> EPDIRPCGRSLVIISTLDGRIAALDPENHGKKQWDLDVGSGSLVSSSLSKPEVFGNKMIIPSLDGDLFQWDRDRESMETVPFTVESLLESSYKFGDDVVLVGGKSLTTYGLSAYSGKVRYICSALGCRQWDNDEMEQEEDILLLQRTQKTVRAVGPRSGNEKWNFSVGHFELRYIPDMETRAGFIE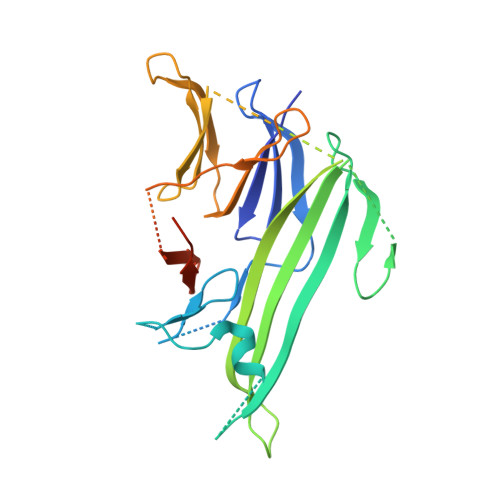STLKPSGNKEQSKIISDVEEQEAVMMDTVIKVSVADWKVMAFNKKGGHLEWEYQFSTPIASAWLVKDGKVIPISLFDDTSYAPNDGVLEDEEDIVEAARGATENSVYLGMYRGQLYLQSSVRISEKFPTSPKALESVSSE> APDTSVSNKQNFSTDVIYQIFTDRFSDGNPANNPTGAAFDGTCTNLRLYCGGDWQGIINKINDGYLTGMGVTAIWISQPVENIYSIINYSGVNNTAYHGYWARDFKKTNPAYGTIADFQNLIAAAHAKNIKVIIDFAPNHTSP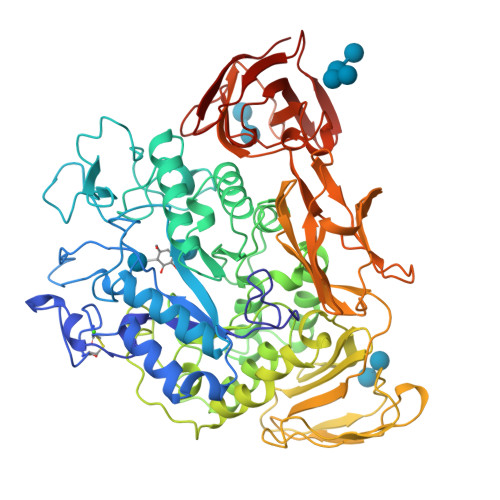ASSDQPSFAENGRLYDNGTLLGGYTNDTQNLFHHNGGTDFSTTENGIYKNLYDLADLNHNNSTVDVYLKDAIKMWLDLGIDGIRMDAVKHMPFGWQKSFMAAVNNYKPVFTFGEWFLGVNEVSPENHKFANESGMSLLDFRFAQKVRQVFRDNTDNMYGLKAMLEGSAADYAQVDDQVTFIDNHDMERFHASNANRRKLEQALAFTLTSRGVPAIYYGTEQYMSGGTDPDNRARIPSFSTSTTAYQVIQKLAPLRKCNPAIAYGSTQERWINNDVLIYERKFGSNVAVVAVNRNLNAPASISGLVTSLPQGSYNDVLGGLLNGNTLSVGSGGAASNFTLAAGGTAVWQYTAATATPTIGHVGPMMAKPGVTITIDGRGFGSSKGTVYFGTTAVSGADITSWEDTQIKVKIPAVAGGNYNIKVANAAGTASNVYDNFEVLSGDQVSVRFVVNNATTALGQNVYLTGSVSELGNWDPAKAIGPMYNQVVYQYPNWYYDVSVPAGKTIEFKFLKKQGSTVTWEGGSNHTFTAPSSGTATINVNWQP>SVKERTEQIEHILKSSVVKVAYGSSNPKRSEPDLNILKDLIDSNYVVFDVLLQFLTHQDPVVTAAAAQVYIRRAYRAYTIGDIRVHEGVTVPIVEWKFQLPSAAFSTFPTVKSKMGMNRAVSVSDLSYVANSQSSPLREGILMAVDHLDDVDEILSQSLEVIPRHQSSSNGPAPDRSGSSASLSNVANVCVASTEGFESEEEILVRLREILDLNKQELINASIRRITFMFGFKDGSYPKYYTFNGPNYNENETIRHIEPA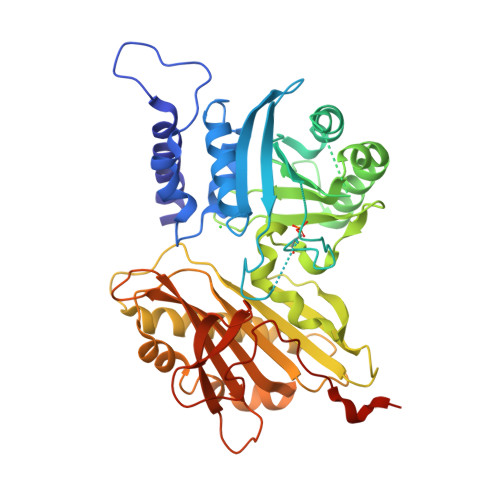LAFQLELGRLSNFNIKPIFTDNRNIHVYEAVSKTSPLDKRFFTRGIIRTGHIRDDISIQEYLTSEANRLMSDILDNLEVTDTSNSDLNHIFINFIAVFDISPEDVEAAFGGFLERFGKRLLRLRVSSAEIRIIIKDPQTGAPVPLRALINNVSGYVIKTEMYTEVKNAKGEWVFKSLGKPGSMHLRPIATPYPVKEWLQPKRYKAHLMHHHHHH[2x]>[8x]MPFIYRRRVQFYETDAQGIVHHSNYFRYFEEARGEFLRSKG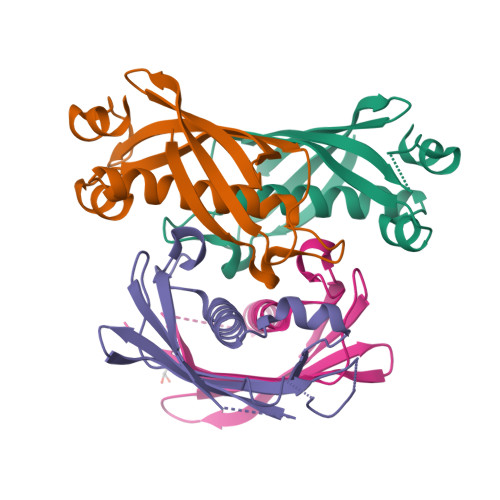FPYSKMRDMGLEVVLLNAYCEYKKPLFYDDVFEVHLNLEELSRFTFTFSYIVFKEDIAVAKANTKHCMVKNGKIVSIPKEVLEVLKD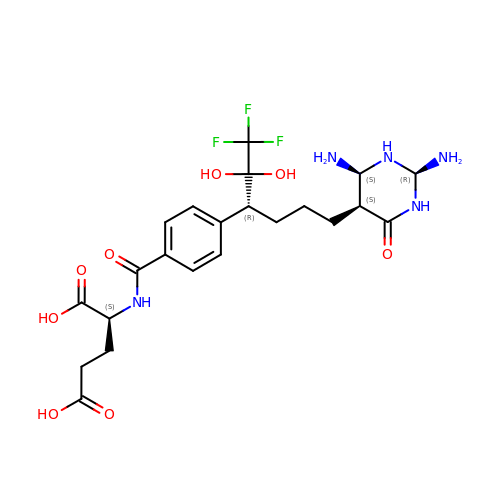N-{4-[(1R)-4-[(2R,4R,5S)-2,4-DIAMINO-6-OXOHEXAHYDROPYRIMIDIN-5-YL]-1-(2,2,2-TRIFLUORO-1,1-DIHYDROXYETHYL)BUTYL]BENZOYL}-D-GLUTAMIC ACID | C22 H30 F3 N5 O8 | KOLDLUFBEMUZIM-YNPGLMGXSA-N> MEPHSLRYNLTVLSWDGSVQSGFLTEVHLDGQPFLRCDRQKCRAKPQGQWAEDVLGNKTWDRETRDLTGNGKDLRMTLAHIKDQKEGLHSLQEIRVCEIHEDNSTRSSQHFYYDGELFLSQNLETKEWTMPQSSRAQTLAMNVRNFLKEDAMKTKTHYHAMRADCLQELRRYLKSGVILRRTVPPMVNVTRSEASEGNITVTCRASGFYPWNITLSWRQDGVSLSHDTQQ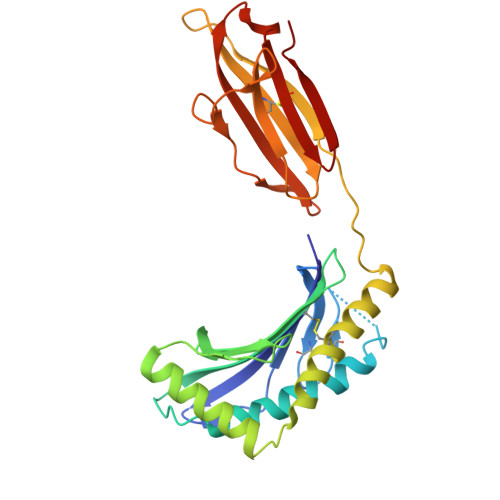WGDVLPDGNGTYQTWVATRICQGEEQRFTCYMEHSGNHSTHPVPS> MTVRLDQQTRQRLQDIVKGGYRSANAAI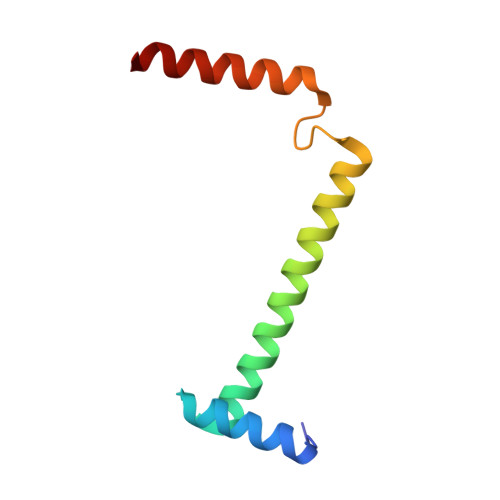VDAINKRWEALHDEQLDAAYAAAIHDNPAYPYESEAERSAARARRNARQQRSA> MAQSVTADPSPPITDTNKLNKYSSRITEPKSQGGSQAILHGVGLSDDDLLKPQIGISSVWYEGNTCNMHLLKLSEAVKEGVENAGMVGFRFNTIGVSDAISMGTRGMCFSLQSRDLIADSIETVMSAQWYDGNISIPGCDKNMPGTIMAMGRLNRPGIMVYGGTIKPGHFQDKTYDIVSAFQSYGEFVSGSISDEQRKTVLHHSCPGAGACGGMYTANTMASAIEAMGMSLPYSSSIPAEDPLKLDECRLAGKYLLELLKMDLKPRDIITPKSLRNAMVSVMALGGSTNAVLHLIAIARSVGLELTLDDFQKVSDAVPFLADLKPSGKYVMEDIHKIGGTPAVLRYLLELGLMDGDCMTVTGQTLAQNLENVPSLTEGQEIIRPLSNPIKETGHIQILRGDLAPDGSVAKITGKEGLYFSGPALVFEGEESMLAAISADPMSFKGTVVVIRGEGPKGGPGMPEMLTPTSAIMGAGLGKECALLTDGRFSGGSHGFWVGHICPEAQEGGPIGLIKNGDIITIDIGKKRIDTQVSPEEMNDRRKKWTAPAYKVNRGVLYKYIKNVQSASDGCVTDE

Dihydroxy acid dehydratase (DHAD) is the third enzyme in the plant branched-chain amino acid biosynthetic pathway and the target for commercial herbicide development. We have previously reported the discovery of fungal natural product aspterric acid (AA) as a submicromolar inhibitor of DHAD through self-resistance gene directed genome mining. Here, we reveal the mechanism of AA inhibition on DHAD and the self-resistance mechanism of AstD, which is encoded by the self-resistance gene astD. Our structural and kinetic analysis of the mutant AthDHADs has validated the hypothesis that larger hydrophobic amino acids surrounding the active-site entrance enhance resistance to AA.

To determine if small-to-large amino acid mutations at these hydrophobic residues can decrease active site volume and increase resistance to AA, we generated multiple mutations at V496, V497, and I177 in AthDHAD followed by kinetic and structural characterizations. The substitutions of V496L and V497I may push the loop where G490 is located toward the center of the channel. To probe the acquired resistance mechanism of AthDHAD mutants, we determined the crystal of AthDHAD–I177F (2.45 Å), AthDHAD–V178W (1.77 Å), AthDHAD–V496W (1.59 Å), and AthDHAD–V497F (1.87 Å). In the crystal structures of I177F, V178W, V496W, and V497F, the occupancy of [2Fe–2S] cluster is 0.64, 0.72, 0.63, and 0.77, respectively. The overall structures of the AthDHAD mutants I177F, V178W, V496W, and V497F displayed high similarity with the wild-type AthDHAD, with the RMSD of 0.123 Å (888 core Cα atoms), 0.275 Å (994 core Cα atoms), 0.142 Å (1,034 core Cα atoms), and 0.283 Å (994 core Cα atoms), respectively. The obvious difference was in loop 490–497, which forms the side wall at the narrowest point of the substrate channel. For example, in the V496W structure, the side chain of W496 induced the loop 489–493 move toward V178, which made the chamber entrance narrower and might block AA to access the active site.At the heart of the spliceosome is pre-mRNA processing factor 8 (Prp8), a large (approximately 270 kDa) and highly conserved protein. Prp8 helps generate mature mRNA by coordinating critical rearrangements at the catalytic core of the spliceosome. The intein-containing precursor undergoes protein splicing, a process that excises the intein and ligates the flanking sequences, called exteins, to form the functional protein. The intein is also found at a highly conserved site at the center of Prp8 and thus is at the core of the spliceosome.

To further understand the mode of zinc binding, we turned to crystal soaking in zinc acetate. We determined the crystal structure of the Cne Prp8 intein in complex with Zn2+ at 1.85 Å resolution. Compared with the native form, the complex does not show significant conformational changes, as is reflected by a small overall RMSD (0.17 Å) between the 2 structures. There are 6 molecules per asymmetric unit cell. All 6 molecules bind 1 Zn2+ at their C terminus with the terminal asparagine (N171), and 3 molecules bind an additional Zn2+ at their N terminal C1. The Zn2+ at the C terminus is coordinated by the main chain carboxyl oxygen of the N171 and 2 water molecules. Binding at this site induces an alternative conformation for the main chain peptide carboxyl group to provide a ligand for Zn2+. This alternative conformation is not seen in the native structure. Zn2+ binding to either of these 2 catalytic residues prevents Prp8 protein splicing.

>[6x]MGKACLQNGTRLLRADGSEVLVEDVQEGDQLLGPDGTSRTASKIVRGEERLYRIKTHEGLEDLVCTHNHILSMYKERFGREGAHSPSAGTSLTESHERVDVTVDDFVRLPQQEQQKYKLFRSTDFVRREQPSASKLATLLHINSIELEEEPTKWSGFVVDKDSLYLRYDYLVLHNSLEHHHHHH> MLDNLAVHPEQLPPRPWITLKERDQILPSASFTVMCYNVLCDKYATRQLYGYCPSWALNWEYRKKGIMEEIVNCDADIISLQEVETEQYFTLFLPALKERGYDGFFSPKSRAKIMSEQERKHVDGCAIFFKTEKFTLVQKHTVEFNQVAMANSDGSEAMLNRVMTKDNIGVAVVLEVHKELFGAGMKPIHAADKQLLIVANAHMHWDPEYSDVKLIQTMMFVSEVKNILEKASSRPGSPTADPNSIPLVLCA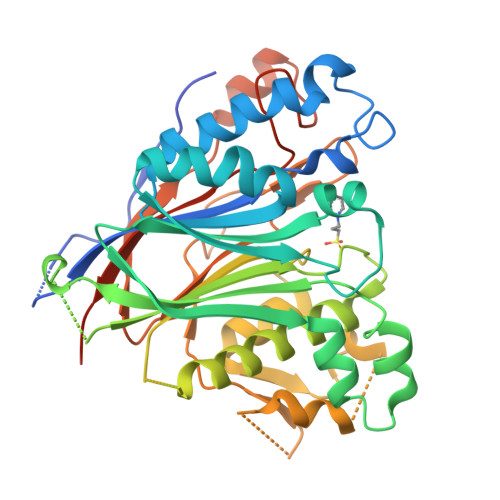DLNSLPDSGVVEYLSNGGVADNHKDFKELRYNECLMNFSCNGKNGSSEGRITHGFQLKSAYENNLMPYTNYTFDFKGVIDYIFYSKTHMNVEGVLGPLDPQWLVENNITGCPHPHIPSDHFSLLTQLELHPPLLPLVNGVHLPNRR> QLNDIISPHKDVHESEFYRYMNNSFAQDLKMKQLMNWCLIRALRKLEIKNSQNKSESRKITLTILKDFVRDIRKGSHDIDWXXXXXXXXXXXXXXXXXXXXXXXXXXXXXXXXXXXXXXX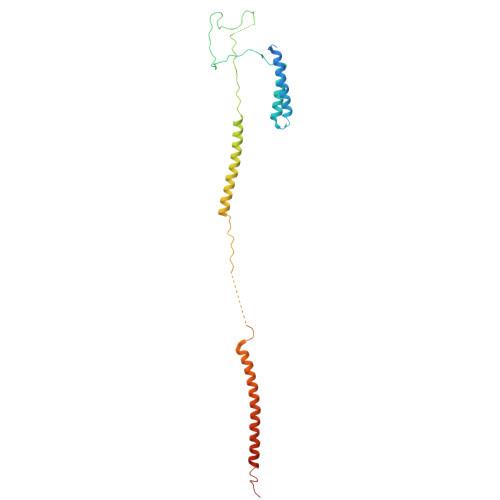XXXPPIKLAKIPNEKNIQNKENAKILEEKIKTIKNEIEQWSKDLSDVKIPSYELPKSQTSIVKLPDNLQLTATTKESIHSDFQKRVDGLQETTRLLKSSSILLNETAGMKLQRLNGCIVKKRPEDKNSTK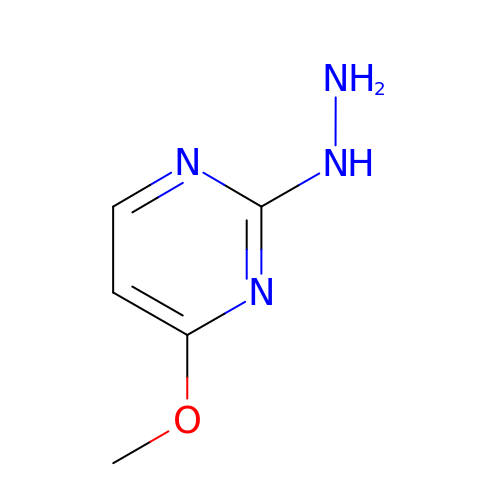2-hydrazinyl-4-methoxypyrimidine | C5 H8 N4 O | HXQPYFMXCAIHAB-UHFFFAOYSA-N9-(7-{[amino(iminio)methyl]amino}-5,6,7-trideoxy-beta-D-ribo-heptofuranosyl)-9H-purin-6-amine 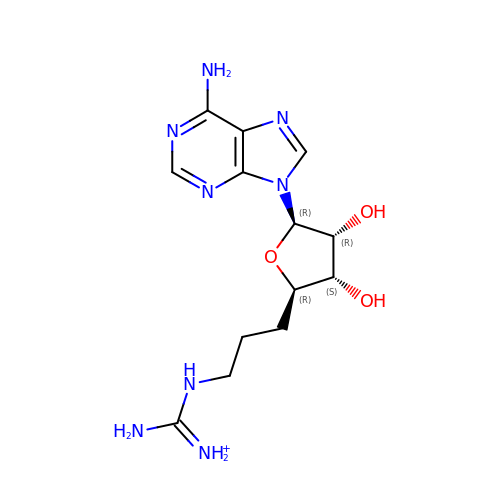| C13 H21 N8 O3 | NGQAXJZDWQDSQY-WOUKDFQISA-O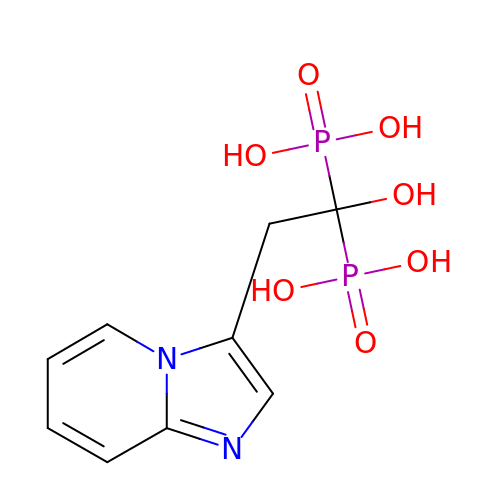(1-HYDROXY-2-IMIDAZO[1,2-A]PYRIDIN-3-YLETHANE-1,1-DIYL)BIS(PHOSPHONIC ACID) | C9 H12 N2 O7 P2 | VMMKGHQPQIEGSQ-UHFFFAOYSA-N> GMSETITFPPLMTGEAAGPGQDPFDLACQKAELGVDAGLVVYELGTDVLRAALVLAPEVPLAKAMAMLPVCGVGFQNALGALAPPEVAVHLDWNGALRINGARCGRLRIAASTDDPDTQPDWLVVGLDLPLWPEGDGGETPDETALYAEGCADVAAPRLLESWAR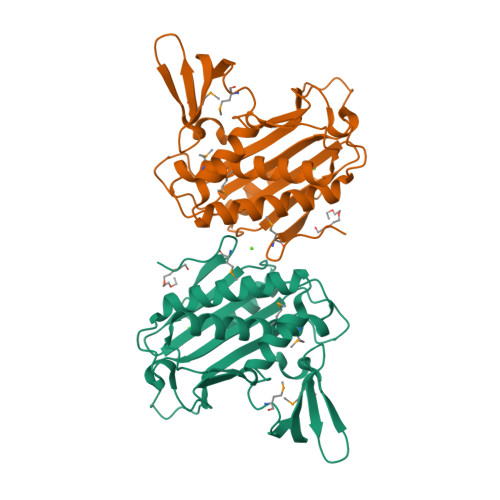HCLHWINRWDEGELETIHGEWRGLAHGMGEARTEAGRSGTFLGVDEDFGMLLRDETTTHLIPLTTVLVQD>MTPDIILQRTGIDVRAVEQGDDAWHKLR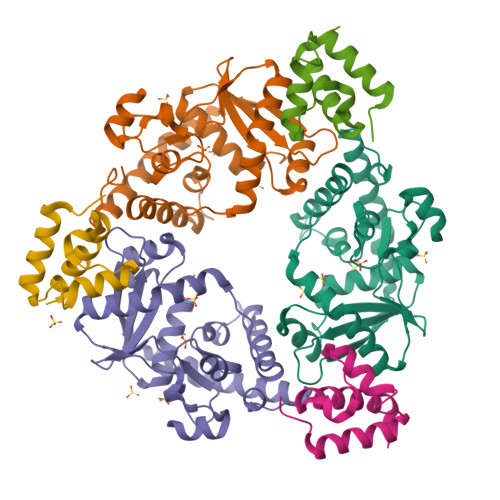LGVITASEVHNVIAKPRSGKKWPDMKMSYFHTLLAEVCTGVAPEVNAKALAWGKQYENDARTLFEFTSGVNVTESPIIYRDESMRTACSPDGLCSDGNGLELKCPFTSRDFMKFRLGGFEAIKSAYMAQVQYSMWVTRKNAWYFANYDPRMKREGLHYVVIERDEKYMASFDEIVPEFIEKMDEALAEIGFVFGEQWR[3x];>ITPVNDETMQEINTLLIALDKTWDDDLLPLCSQIFRRDIRASSELTQAEAVKALGFLKQKAAEQKVA[3x]>[4x]MSTGTSNLVAVEPGAIREDTPPGSVIQYSDYELDHSSPFAGGVAWIEGEFLPAEDAKISIFDTGFGHSDLTYTVAHVWHGNIFRLGDHLDRLLDGARKLR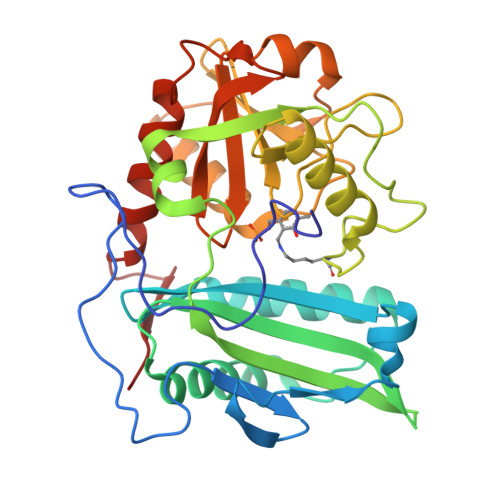LDAGYTKDELADITKQCVSMSQLRESFVNLTVTRGYGKRRGEKDLSKLTHQVYIYAIPYLWAFPPAEQIFGTTAIVPRHVRRAGRNTVDPTIKNYQWGDLTAASFEAKDRGARTAILLDSDNCVAEGPGFNVCIVKDGKLASPSRNALPGITRKTVFEIADQMGIEATLRDVTSHELYDADELMAVTTAGGVTPINSLDGEAIGNGAPGPMTVAIRDRFWALMDEPGPLIEAIEY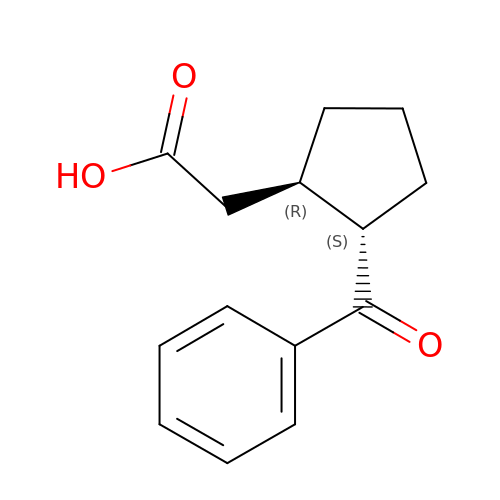[(1R,2S)-2-(benzenecarbonyl)cyclopentyl]acetic acid | C14 H16 O3 | NMNCOSWJMSHIOO-NEPJUHHUSA-N(10R,12S)-12-[(1R)-1-hydroxy-2-({[3-(propan-2-yl)phenyl]methyl}amino)ethyl]-17-(methoxymethyl)-10-methyl-2,13-diazabicyclo[13.3.1]nonadeca-1(19),15,17-trien-14-one 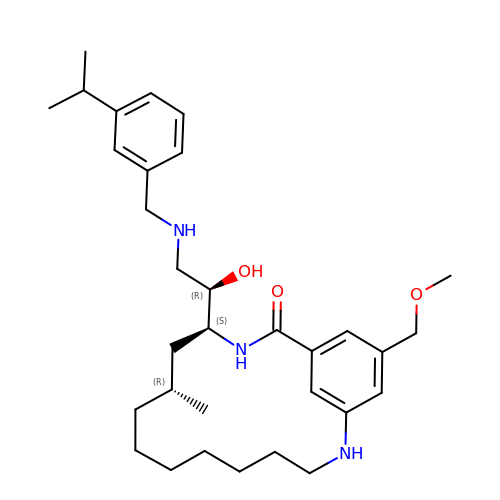| C32 H49 N3 O3 | UGCIUWIDOWOQSA-XGJRVREISA-N> DRASKI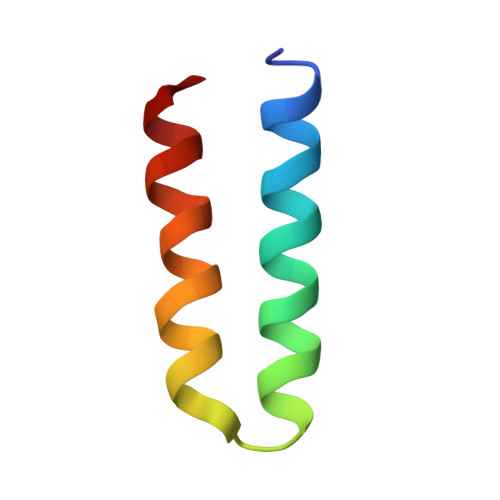EQIQKLAKYAISALNYEDLPTAKDELTKALDLLNSI Precise division over and capture of the forespore-destined chromosome requires RefZ, a TetR family DNA-binding protein conserved across the genus Bacillus. RefZ binds to five nearly palindromic DNA motifs (RBMs), two on each chromosomal arm and one near oriC. Second, artificially induced expression of RefZ during vegetative growth disrupts Z ring assembly and inhibits cell division. We propose that RBM-bound RefZ complexes function as a developmentally regulated nucleoid occlusion system for fine-tuning the position of the septum relative to the chromosome during sporulation.

RefZ-His6 was purified and crystallized, and the structure was solved using single-wavelength anomalous dispersion (SAD) phasing at a resolution of 2.6 Å. RefZ crystallized as a homodimer with one molecule in the asymmetric unit of a P41212 crystal lattice. Each RefZ subunit is composed of 10 α-helices connected by loops and turns. Similar to other structurally characterized TetR family proteins, α1, α2, and α3 comprise the DNA-binding helix-turn-helix (HTH) domain and α4 to α10 comprise the regulatory domain. There are two major regions for dimerization contacts. Helices α7, α8, α9, and α10 form regulatory domain contacts with α7′, α8′, α9′, and α10′; α8, α10, α8′, and α10′ form a four-helix dimerization motif. A second interface is formed by α6 and α6′ at the junction between the regulatory and DNA-binding domains. Although the crystallization conditions included RBM-containing DNA, we observed no DNA in the crystal structure. In fact, the HTH DNA-binding domain is involved in extensive crystal-packing interactions, likely precluding DNA binding within the crystal lattice. In the RefZ structure (unbound from DNA), there is no obvious ligand binding pocket in the α5-to-α7 regulatory region; therefore, its affinity with DNA is unlikely to be regulated in this manner.

> MKVSTKDKIIESAVMLFNQKGFSGTSVREIAKSADVNVAHISYYFKGKGGLMEHLVSEFYEGYSKTLETAASNISTQSTQEQLLQLVFDILSYQHNHRQLTRFVYREVTIDSTLIREIMSTYLMKEKYIFQLIIEEGEKQREYLTLPLPHFILQLKSLLMMPYLQPQYISEVLYMQPHEPYFYKMYFEEIKIWIRSVFRTGDVALTN> GPLGSMNHQQQQQQQKAGEQQLSEPEDMEMEAGDTDDPPRITQNPVINGNVALSDGHNTAEEDMEDDTSWRSEATFQFTVERFSRLSESVLSPPCFVRNLPWKIMVMPRFYPDRPHQKSVGFFLQCNAESDSTSWSCHAQAVLKIINYRDDEKSFSRRISHLFFHKENDWGFSNFMAWSEVTDPEKGFIDDDKVTFEVFVQADAPHGVAWDSKKHTGYVGLKNQGATCYMNSLLQTLFFTNQLRKAVYMMPTEGDDSSKSVPLALQRVFYELQHSDKPVGTKKLTKSFGWETLDSFMQHDVQELCRVLLDNVENKMKGTCVEGTIPKLFRGKMVSYIQCKEVDYRSDRREDYYDIQLSIKGKKNIFESFVDYVAVEQLDGDNKYDAGEHGLQEAEKGVKFLTLPPVLHLQLMRFMYDPQTDQNIKINDRFEFPEQLPLDEFLQKTDPKDPANYILHAVLVHSGDNHGGHYVVYLNPKGDGKWCKFDDDVVSRCTKEEAIEHNYGGHDDDLSVRHCTNAYMLVYIRESKLSEVLQAVTDHDIPQQLVERLQEEKRIEAQKRKERQEAHLYMQVQIVAEDQFCGHQGNDMYDEEKVKYTVFKVLKNSSLAEFVQSLSQTMGFPQDQIRLWPMQARSNGTKRPAMLDNEADGNKTMIELSDNENPWTIFLETVDPELAASGATLPKFDKDHDVMLFLKMYDPKTRSLNYCGHIYTPISCKIRDLLPVMCDRAGFIQDTSLILYEEVKPNLTERIQDYDVSLDKALDELMDGDIIVFQKDDPENDNSELPTAKEYFRDLYHRVDVIFCDKTIPNDPGFVVTLSNRMNYFQVAKTVAQRLNTDPMLLQFFKSQGYRDGPGNPLRH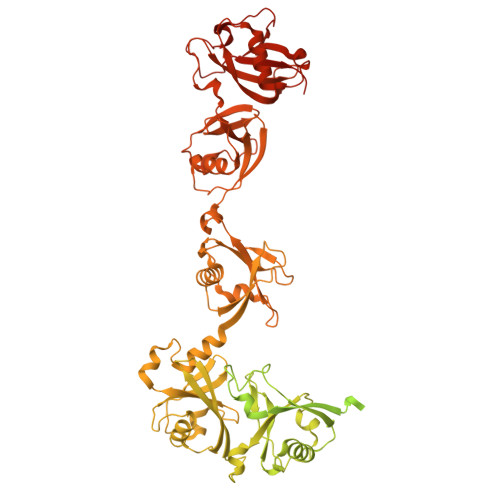NYEGTLRDLLQFFKPRQPKKLYYQQLKMKITDFENRRSFKCIWLNSQFREEEITLYPDKHGCVRDLLEECKKAVELGEKASGKLRLLEIVSYKIIGVHQEDELLECLSPATSRTFRIEEIPLDQVDIDKENEMLVTVAHFHKEVFGTFGIPFLLRIHQGEHFREVMKRIQSLLDIQEKEFEKFKFAIVMMGRHQYINEDEYEVNLKDFEPQPGNMSHPRPWLGLDHFNKAPKRSRYTYLEKAIKIHN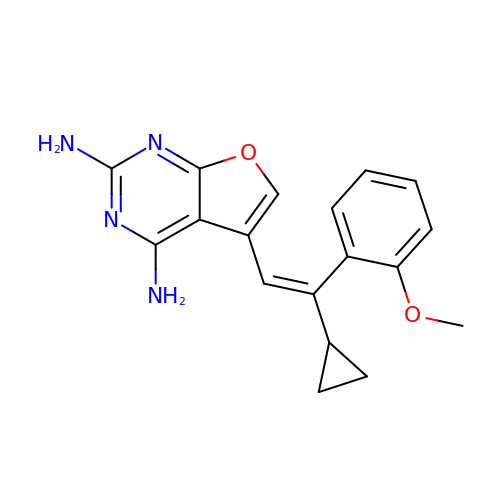5-[(E)-2-cyclopropyl-2-(2-methoxyphenyl)ethenyl]furo[2,3-d]pyrimidine-2,4-diamine | C18 H18 N4 O2 | PUOLMVSSUQSKAQ-MDWZMJQESA-N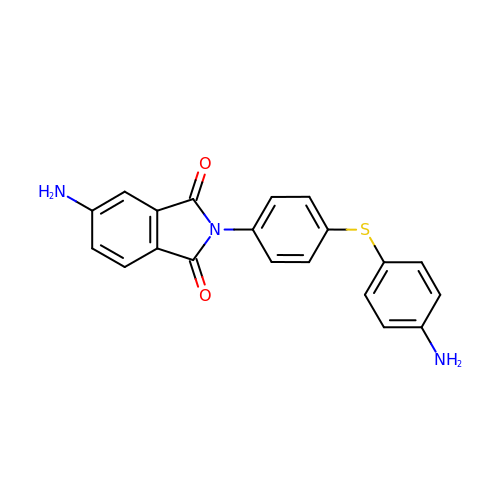5-AMINO-2-{4-[(4-AMINOPHENYL)SULFANYL]PHENYL}-1H-ISOINDOLE-1,3(2H)-DIONE | C20 H15 N3 O2 S | FQQVTDIBUYSVHM-UHFFFAOYSA-N> GGGSAAGKKVVYSTFGAQIPFFNRIGEGAKAQATVRRLDFDISTSEIDPGKQIDSIDNAVAQQPDGLIVSPIDGSALVPTIKGAVEDGVPVILLADGLSEDVGQLSFVGSDFAEIGRLKATYIADRLGDGGTVAMVN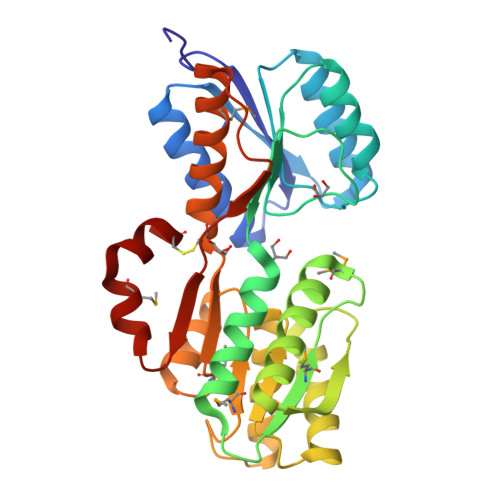GTRGMSFVEEQGEAAREVFEERGIEIVDDVYTKAITPDEGLTATQNILTRHSDVGAIYYSGDDGALGGIRAIAARNIAPGKIMVVGTDANEGALAAVRAGTMALTVSQCAYEQGGIAIDVMADYLETGKKPDRRIFTPVIEIDTETIDRVMSGAAWERCENH> MDKPIIAYLSDIGNHDEAHALGKGLIKTIAPGAEIVDITHQVTPFDVREGGLYLQDVPASFPANTVIAAYVYPETGTSTRTVVVRNEKGQLLVAPN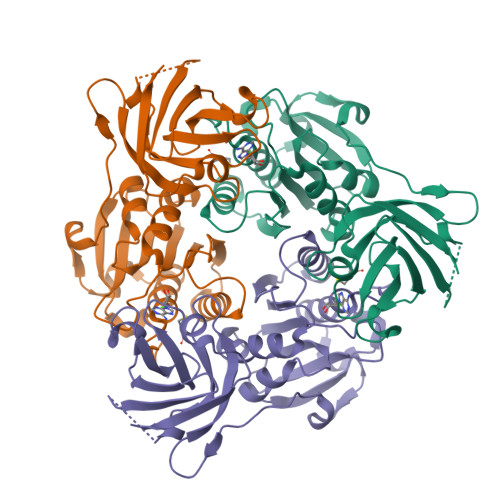NGLLTWALKAVPAVEAWEVTSPDVMNQPVTPTWYGKDVVVACGAHLAAGVAPSAVGPKIDVAKLVTLPTTPAVQLGDGSVRGEVVRIDKAFGNVWTNISLDALSGGGALDGKTLQVTAEGLSVEIPYYATFGEVPIGEPLVYNNSRGKVALGLNQGSFLERYGVAAGDTVTIGLV>[2x]MDPKFQRVALSDGHFIPVLGFGTYAPEEVPKSKAMEATKIAIDAGFRHIDSAYFYKNEKEVGLAIRSKIADGTVKREDIFYTSKLWCTFHRPELVRPSLEDSLKNLQLDYVDLYIIHFPTALKPGVEIIPTDEHGKAIFDTVDICATWEAMEKCKDAGLAKSIGVSNFNRRQLEMILNKPGLKYKPVCNQVECHPYLNQGKLLEFCKSKGIVLVAYSALGSHREPEWVDQSAPVLLED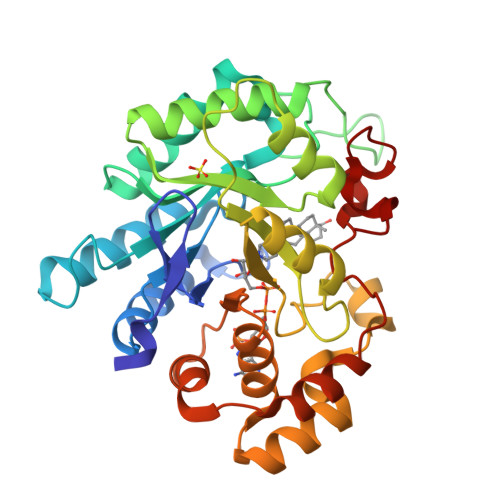PLIGALAKKHQQTPALIALRYQLQRGIVVLAKSFTEKRIKENIQVFEFQLPSEDMKVIDSLNRNFRYVTADFAIGHPNYPFSDEY Mycobacterium tuberculosis, the etiological agent of TB, possesses a cholesterol catabolic pathway implicated in pathogenesis. This pathway includes an iron-dependent extradiol dioxygenase, HsaC, that cleaves catechols. As in the aerobic bacterial degradation of other steroids, the core 4-ringed structure is degraded via opening of ring B with concomitant aromatization of ring A. The resulting phenolic metabolite is hydroxylated, yielding a catechol, 3,4-dihydroxy-9,10-seco-nandrost-1,3,5(10)-triene-9,17-dione (DHSA). HsaC catalyzes the meta-cleavage of DHSA to produce 4,9-DSHA (4,5-9,10-diseco-3-hydroxy-5,9,17-trioxoandrosta-1(10),2-diene-4-oic acid; Figure 1). The overall fold of HsaC is that of a two-domain type I extradiol dioxygenase, with the structure most closely resembling that of BphC (rmsd of 1.16 Å for the 275 common Cα atoms). The active site is located within the central cavity of the slightly larger C-terminal domain, with the catalytically essential mononuclear Fe2+ ligated by His145, His215 and Glu266.

Crystal structures of HsaC were obtained in its substrate-free form and in complex with DHSA at resolutions of 2.0 and 2.2 Å, respectively. In crystals of HsaC soaked anaerobically with DHSA, the active site cavity of each molecule in the asymmetric unit contained additional electron density that corresponds to the steroid metabolite, DHSA. Remarkably, DHSA binds in different modes in each of the molecules, with the catecholic ring coordinating the Fe in bidentate and monodentate manners in molecules A and B, respectively. The asymmetric, bidentate binding of the catecholic moiety in molecule A corresponds to that which has been reported in other extradiol dioxygenase:substrate complexes. Briefly, the proximal hydroxyl (O4) of the catecholic ring binds the Fe in the site trans to His145 and the distal hydroxyl (O3) binds trans to His215, displacing the two water molecules in the resting state enzyme. In molecule B, the catecholic ring is bound to the iron in a monodentate manner via the 4-hydroxyl (proximal) group with an O4-Fe distance of 2.8 Å. With respect to its conformation in molecule A, the catecholic moiety of DHSA is rotated 60° clock-wise around the ligand's C6–C7 bond such that the O3 hydroxyl is 3.7 Å away from the Fe. In contrast to the different binding modes of the catecholic ring in the two molecules, the bicycloalkanone moiety of the bound DHSA occupies strikingly similar conformations in the two complexes, suggesting that this moiety is a major determinant in the binding of the substrate. More precisely, the bicycloalkanone moiety occupies a largely hydrophobic portion of the substrate-binding site, contacting Leu174, Leu190, Leu205, Val 214, and Phe294. The structure of the monodentate-bound HsaC:DHSA complex was unexpected, but potentially provides insights into the initial substrate-binding steps of extradiol dioxygenases.

>MSIRSLGYLRIEATDMAAWREYGLKVLGMVEGKGAPEGALYLRMDDFPARLVVVPGEHDRLLEAGWECANAEGLQEIRNRLDLEGTPYKEATAAELADRRVDEMIRFADPSGNCLEVFHGTALEHRRVVSPYGHRFVTGEQGMGHVVLSTRDDAEALHFYRDVLGFRLRDSMRLPPQMVGRPADGPPAWLRFFGCNPRHHSLAFLPMPTSSGIVHLMVEVEQADDVGLCLDRALRRKVPMSATLGRHVNDLMLSFYMKTPGGFDIEFGCEGRQVDDRDWIARESTAVSLWGHDFTVGARG[2x]> SSESTTFIVDVSPSMMKNNNVSKSMAYLEYTLLNKSKKSRKTDWISCYLANCPVSENSQEIPNVFQIQSFLAPVTTTATIGFIKR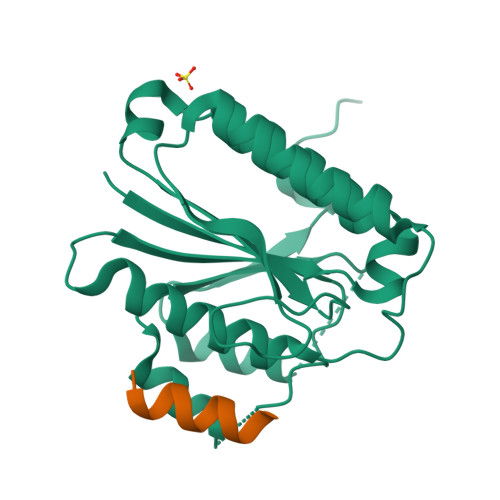LKQYCDQHSHDSSNEGLQSMIQCLLVVSLDIKQQFQARKILKQIVVFTDNLDDLDITDEEIDLLTEELSTRIILIDCGKDTQEERKKSNWLKLVEAIPNSRIYNMNELLVEITS;> NSKLLSLLRSKT MalT is a bacterial STAND that controls the Escherichia coli maltose system. It bears all the hallmarks of STAND family proteins with a tripartite domain architecture, comprising an N-terminal nucleotide-binding and oligomerization (NOD) module, a superhelical peptide repeats (SUPR)-type sensor domain, and an effector domain that confers DNA-binding activity. The other two MalT repressors are MalY a pyridoxal 5’-phosphate (PLP)-dependent dimeric enzyme and Aes, an enzyme with acetyl esterase activity. MalT is known to cycle between two states, a monomeric ADP-bound resting form, and an oligomeric ATP-bound active form.

Here we report the cryogenic electron microscopy (cryo-EM) structure of an inhibitory complex consisting of MalT and MalY, which reveals a heterotetrameric assembly with a stoichiometry of 2:2 between two proteins. After 3D reconstruction and 3D classification, a subset of 176,969 particles were used for final refinement, yielding a map with a global resolution of 2.94 Å. The overall structure of the MalT-MalY complex is shaped like the capital letter “H”. In the complex, MalY forms a homodimer with each of its subunits bound by one cofactor PLP. The MalT structure that is well defined corresponds to the four N-terminal domains of the protein: the nucleotide-binding domain (NBD, residue 1–181), the helical domain (HD, residue 182–248), the winged-helix domain (WHD, residue 249–336), and the arm domain (residue 337–423). Consistently, a cryo-EM density corresponding to an ADP molecule was found between the NBD, HD, and WHD. Notably, intramolecular interactions between the NBD and WHD of MalT are directly mediated by the N-terminal segment of NBD, indicating a critical role of this segment in maintaining MalT autoinhibition. The MalT α8 helix and its N-terminal segment dominate the interactions via packing against one side of the PLP-binding domain of MalY. MalT R173 at the C-terminal side of α8 forms a bidentate salt bond with MalY D182 and E185 and makes van der Waals packing against MalY C181. By analyzing different interaction interfaces contributing to MalT inhibition, we found that MalY binds to one oligomerization surface of MalT, thereby inhibiting MalT activation by blocking oligomerization.

>[2x]MFDFSKVVDRHGTWCTQWDYVADRFGTADLLPFTISDMDFATAPCIIEALNQRLMHGVFGYSRWKNDEFLAAIAHWFSTQHYTAIDSQTVVYGPSVIYMVSELIRQWSETGEGVVIHTPAYDAFYKAIEGNQRTVMPVALEKQADGWFCDMGKLEAVLAKPECKIMLLCSPQNPTGKVWTCDELEIMADLCERHGVRVISDEIHMDMVWGEQPHIPWSNVARGDWALLTSGSKSFNIPALTGAYGIIENSSSRDAYLSALKGRDGLSSPSVLALTAHIAAYQQGAPWLDALRIYLKDNLTYIADKMNAAFPELNWQIPQSTYLAWLDLRPLNIDDNALQKALIEQEKVAIMPGYTYGEEGRGFVRLNAGCPRSKLEKGVAGLINAIRAVR;>MLIPSKLSRPVRLDHTVVRERLLAKLSGANNFRLALITSPAGYGKTTLISQWAAGKNDIGWYSLDEGDNQQERFASYLIAAVQQATNGHCAICETMAQKRQYASLTSLFAQLFIELAEWHSPLYLVIDDYHLITNPVIHESMRFFIRHQPENLTLVVLSRNLPQLGIANLRVRDQLLEIGSQQLAFTHQEANEFFDCRLSSPIEAAESSRICDDVSGWATALQLIALSARQNTHSAHKSARRLAGINASHLSDYLVDEVLDNVDLATRHFLLKSAILRSMNDALITRVTGEENGQMRLEEIERQGLFLQRMDDTGEWFCYHPLFGNFLRQRCQWELAAELPEIHRAAAESWMAQGFPSEAIHHALAAGDALMLRDILLNHAWSLFNHSELSLLEESLKALPWDSLLENPAAAIAIAIIEV[2x]> GPGSTEQAPPVRVLPERIHLHELDPNPPGPESDYRTRWEIPIGLRETDLTPAHCHMHTNPHLLIFGAAKSGKTTIAHAIARAICARNSPQQVRFMLADYRSGLLDAVPDTHLLGAGAINRNSASLDEAVQALAVNLKKRLPPTDLTTAQLRSRSWWSGFDVVLLVDDWHMIVGAAGGMPPMAPLAPLLPAAADIGLHIIVTCQMSQAYKATMDKFVGAAFGSGAPTMFLSGEKQEFPSSEFKVKRRPPGQAFLVSPDGKEVIQAPYIEPPEEVFAAPPSAG;> GPGSMAEMKTDAATLAQEAGNFERISGDLKTQID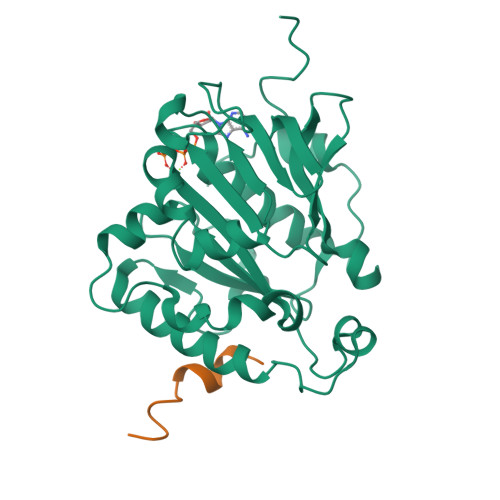QVESTAGSLQGQWRGAAGTAAQAAVVRFQEAANKQKQELDEISTNIRQAGVQYSRADEEQQQALSSQMGF> MEKQNIAVILARQNSKGLPLKNLRKMNGISLLGHTINAAISSKCFDRIIVSTDGGLIAEEAKNFGVEVVLRPAELASDTASSISGVIHALETIGSNSGTVTLLQPTSPLRTGAHIREAFSLFDEKIKGSVVSACPMEHHPLKTLLQINNGEYAPMRHL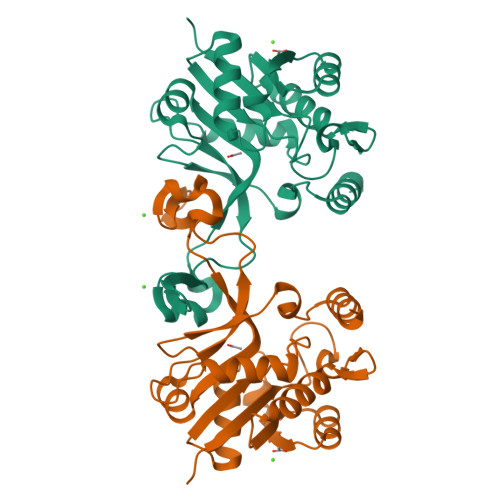SDLEQPRQQLPQAFRPNGAIYINDTASLIANNCFFIAPTKLYIMSHQDSIDIDTELDLQQAENILNHKES>[2x]GLEHCVKIIRQLECSGHIDKNFRQKFLTWYSLRATSQEIRVVKDFIDTFIDDPMALAEQLIDTFDDRVS

The Arabidopsis VEL proteins are accessory proteins that interact with PRC2 to nucleate and propagate silencing at the FLOWERING LOCUS C (FLC) locus, enabling early flowering in spring. Here, we report that VEL proteins contain a domain related to an atypical four-helix bundle that engages in spontaneous concentration-dependent head-to-tail polymerization to assemble dynamic biomolecular condensates. The VEL domain adopts a compact globular fold, consisting of four α-helices in a quasi-antiparallel “up-down-up-down” configuration, each of which contributes to the hydrophobic core, as illustrated by VEL1VEL. Mutations blocking polymerization of this VEL domain prevent Polycomb silencing at FLC.

Noting that most crystal structures of SAM and DIX domains were determined with polymerization-defective mutants, we switched to this approach and thus succeeded in obtaining diffracting crystals of different mutants (including I664D, I575D, and RR>AD) under diverse conditions. We conclude that the VEL head and tail surfaces are defined largely by three key residues, an isoleucine (VIN3I575 or VEL1I664) and two basic residues (VIN3R554,R556 or VEL1R643,K645), that engage in close hydrophobic or electrostatic interactions, respectively, with partner residues from the apposing complementary surface. Indeed, VEL1VEL I664D crystals contain right-handed helical filaments composed of 12 protomers per turn that interact through their head and tail surfaces. Three of these filaments intertwine into a superhelical fiber whose width (∼79 Å) is similar to that of the WT VEL1VEL fibers observed by EM, suggesting correspondence between the superhelical fibers observed by these two methods. The same is true for VEL1 filaments, whereas the VIN3 filaments in the crystals are composed of dimeric VIN3VEL subunits. Clearly, VIN3VEL, but not VEL1VEL, has an intrinsic propensity to undergo domain swapping while forming assemblies during crystallization.>[4x]AGITGTWYNQLGSTFIVTAGADGALTGTYESAVGN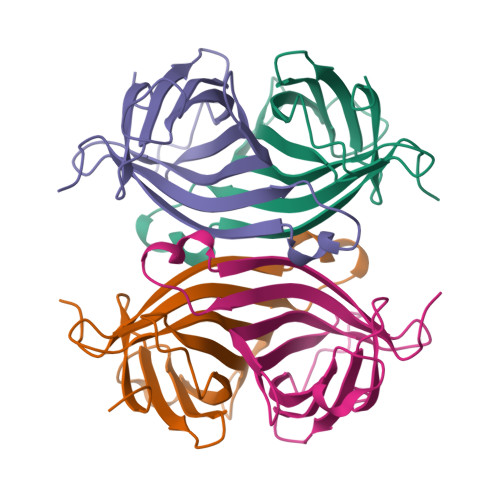AESRYVLTGRYDSAPATDGSGTALGWTVAWKNNYRNAHSATTWSGQYVGGAEARINTQWLLTSGTTEANAWKSTLVGHDTFTKVKPSAASRRRRRRY>[2x]MAGAAAAVAAGAAAGAAAAAVSVAAPGRASAPPPPPPVYCVC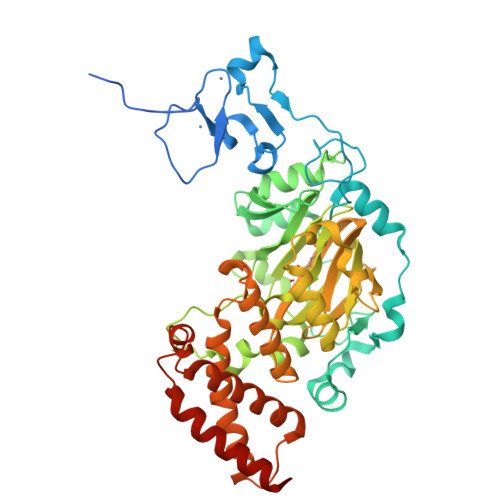RQPYDVNRFMIECDICKDWFHGSCVGVEEHHAVDIDLYHCPNCAVLHGSSLMKKRRNWHRHDYTEIDDGSKPVQAGTRTFIKELRSRVFPSADEIIIKMHGSQLTQRYLEKHGFDVPIMVPKLDDLGLRLPSPTFSVMDVERYVGGDKVIDVIDVARQADSKMTLHNYVKYFMNPNRPKVLNVISLEFSDTKMSELVEVPDIAKKLSWVENYWPDDSVFPKPFVQKYCLMGVQDSYTDFHIDFGGTSVWYHVLWGEKIFYLIKPTDENLARYESWSSSVTQSEVFFGDKVDKCYKCVVKQGHTLFVPTGWIHAVLTSQDCMAFGGNFLHNLNIGMQLRCYEMEKRLKTPDLFKFPFFEAICWFVAKNLLETLKELREDGFQPQTYLVQGVKALHTALKLWMKKELVSEHAFEIPDNVRPGHLIKELSKVIRAIEEENGKPVKSQGI> EEKEQKLQFVLRFGDFEDVISLSKLNVNGSKTTLYSFEN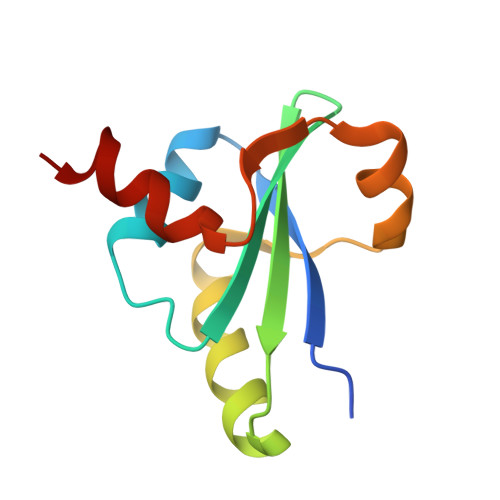RYYLYVDFCNMTDEEVENQLSILLEYATESSISIHRLEEYGKLIISEHALETIKKHFAS>GQDMVSPPPPIADEPLTVNTGIYLIECYSLDDKAETFKVNAFLSLSWKDRRLAFDPVRSGVRVKTYEPEAIWIPAIRFVNVENARDADVVDISVSPDGTVQYLERFSARVLSPLDFRRYPFDSQTLHIYLIVRSVDTRNIVLAVDLEKVGKNDDVFLTGWDIESFTAVVKPANFALEDRLESKLDYQLRISRQYFSYIPNIILPMLFILFISWTAFWSTSYEANVTLVVSTLIAHIAFNILVETNLPKTPYMTYTGAIIFMIYLFYFVAVIEVTVQHYLKVESQPARAASITRASRIAFPVVFLLANIILAFLFFGF[5x]

At present, the best structurally characterized pLGIC is the G. violaceus ligand-gated ion channel (GLIC), of prokaryotic origin. Each subunit consists of an extracellular domain (ECD), predominantly in a β-sandwich fold, and a transmembrane domain (TMD) composed of four helices, labeled M1–M4. However, the GLIC is a pH-gated channel, activated by lowering the pH, with a maximal activation at pH 4 and a pH50 around 5. We instead found that proton activation is a complex multiple loci mechanism, with the key contribution stemming from the coupling interface between the extracellular and transmembrane domain, with E35 acting as a key proton-sensing residue.

In the apical region, the residues either face the solvent (D13, E14, D55, E67, E69, D97), are located at the subunit interface (D49, E75, D136), or are located at the middle of the ECD β-sandwich (E104). The mutants D49N, E75A, D97N, D136N, and D136A display small increases in pH50, but do not meet the criterion for a significant effect. A structural analysis was performed on E26Q, E26A, E35Q, E35A, E67A, E75A, E82Q, E82A, D86A, D88N, D88A, H127N, E181A, and H277Q mutants, by solving their structure at pH 4. All structures were in the apparently open conformation. There are no significant differences, measured as 5-fold over Wt, seen in the backbone Cα residues of any of the resolved structures, with the exception of E35A and E82Q. Additionally, the prediction identified E35, E75, and E243 as gain-of-function locations if mutated, whereas E75 and E243, when mutated, have either no effect or the opposite effect.>SRIVDPKFSSPIVNMTAPVGRDAFLTCVVQDLGPYKVAWLRVDTQTILTIQNHVITKNQRIGIANSEHKTWTM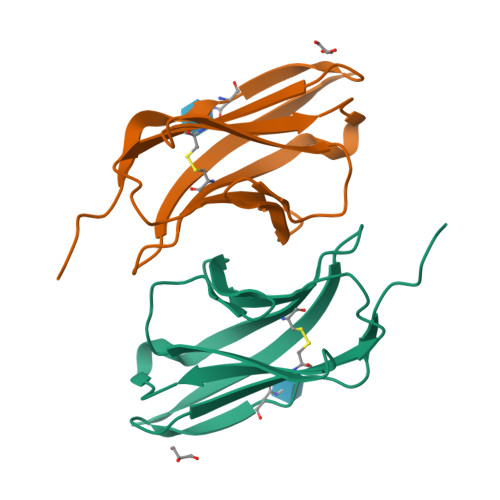RIKDIKESDKGWYMCQINTDPMKSQMGYLDVVVHHHHHH[2x]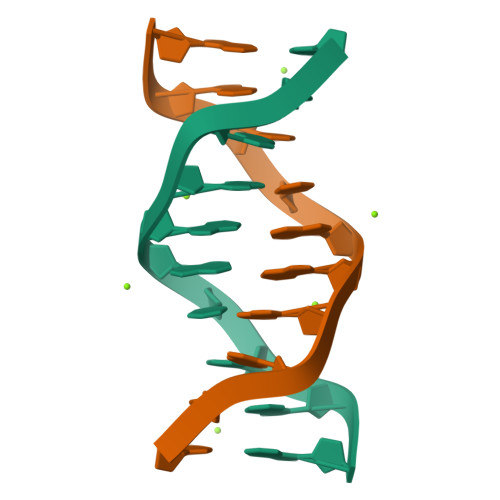> CCAAGATTGG> MKFDKPAGENPIDQLKVVGRPHDRIDGPLKTTGTARYAYEWHEEAPNAAYGYIVGSAIAKGRLTALDTDAAQKAPGVLAVITASNAGVLGKGDKNTARLLGGPTIEHYHQAIALVVAETFEQARAAASLVQAHYRRNKGAYSLADEKQAVNQPPEDTPDKNVGDFDGAFTSAAVKIDATYTTPDQSHMAMEPHASMAVWDGNKLTLWTSNQMIDWCRTDLAKTLKVPVENVRIISPYIGGGFGGKLFLRSDALLAALAARAVKRPVKVMLPRPSIPNNTTHRPATLQHLRIGADQSGKITAISHESWSGNLPGGTPETAVQQSELLYAGANRHTGLRLATLDLPEGNAMRAPGEAPGLMALEIAIDELAEKAGID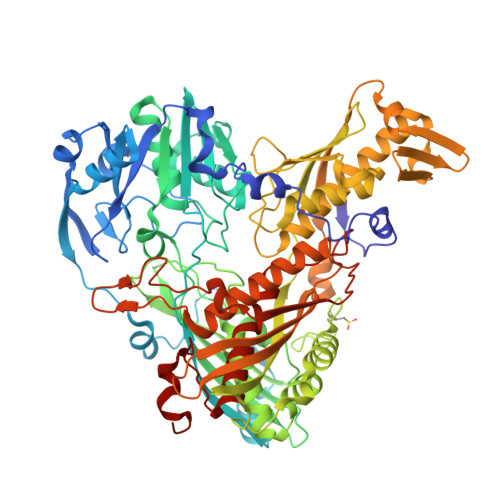PVEFRILNDTQVDPAGPTRCFSRRQLIECLRTGADKFGWKQRNATPGQVRDGEWLVGHGVAAGFRNNLLEKSGARVHLEQNGTVTVETDMTDIGTGSYTILAQTAAEMLGVPLEQVAVHLGDSSFPVSAGSGGQWGANTSTSGVYAACMKLREMIASAVGFDPEQSQFADGKITNGTRSATLHEATAGGRLTAEESIEFGTLSKEYQQSTFAGHFVEVGVHSATGEVRVRRMLAVCAAGRILNPKTARSQVIGAMTMGMGAALMEELAVDDRLGYFVNHDMAGYEVPVHADIPKQEVIFLDDTDPISSPMKAKGVGELGLCGVSAAIANAVYNATGIRVRDYPITLDKLLDKLPDVV4-bromo-2-({[(2-chlorophenyl)carbonyl]amino}methyl)-6-methylphenyl 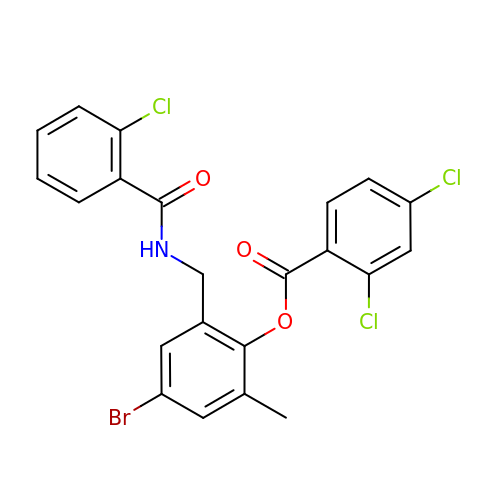2,4-dichlorobenzoate | C22 H15 Br Cl3 N O3 | ZKSVHHXAFVAAHC-UHFFFAOYSA-N>[6x]MVVIGEKFPEVEVKTTHGVIKLPDYFAEQGKWFVLFSHPADFTPVSTTEFYAMQKRVDQFRELGVEPIGLSVDQVCSHIKWMEWIKENLGEEITFPVIADDRGELADKLGMIPSGATITARAVFIVDDKGIIRAIVYYPAEVGRDWDEILRLVKALKVSDEKGVALPHKW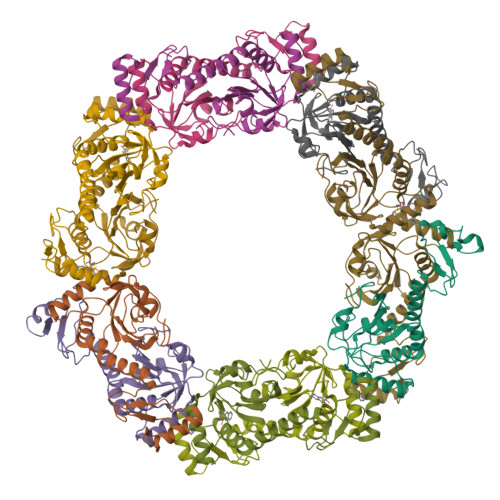PNNELIGDKAIVPPASTVDEVKQREEAKAKGEIESYDWWFSYKKLE;>MVVIGEKFPEVEVKTTHGVIKLPDYFAEQGKWFVLFSHPADCTPVSTTEFYAMQKRVDQFRELGVEPIGLSVDQVFSHIKWMEWIKENLGEEITFPVIADDRGELADKLGMIPSGATITARAVFIVDDKGIIRAIVYYPAEVGRDWDEILRLVKALKVSDEKGVALPHKWPNNELIGDKAIVPPASTVDEVKQREEAKAKGEIESYDWWFSYKKLE[6x]>[2x]MSIKIRDFGLGSDLISLTNKAGVTISFTNLGARIVDWQKDGKHLILGFDSAKEYLEKDAYPGATVGPTAGRIKDGLVKISGKDYILNQNEGPQTLHGGEESIHTKLWTYEVTDLGAEVQVKFSLVSNDGTNGYPGKIEMSVTHSFDDDNKWKIHYEAISDKDTVFNPTGHVYFNLNGDASESVENHGLRLAASRFVPLKDQTEIVRGDIVDIKNT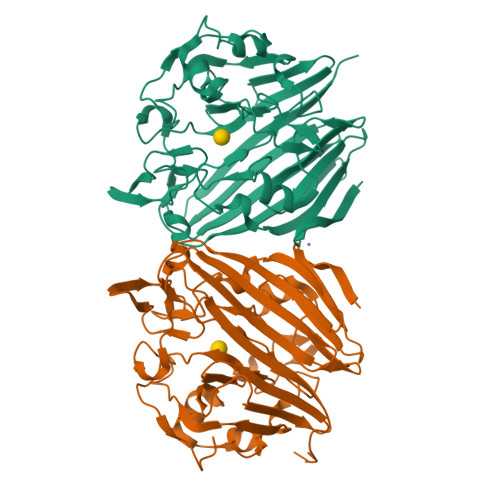DLDFRQEKQLSNAFNSNMEQVQLVKGINHPFLLDQLGLDKEQARLTLDDTSISVFTDQPSIVIFTANFGDLGTLYHEKKQVHHGGITFECQVSPGSEQIPELGDISLKAGEKYQATTIYSLHTKLEHHHHHH>[4x]GSHMLFDFENDQVPSNIHFLNARASIETYTGINGEPSKGLKLAMQSKQHSYTGLAIVPEQPWDWSEFTSASLYFDIVSVGDHSTQFYLDVTDQNGAVFTRSIDIPVGKMQSYYAKLSGHDLEVPDSGDVNDLNLASGLRSNPPTWTS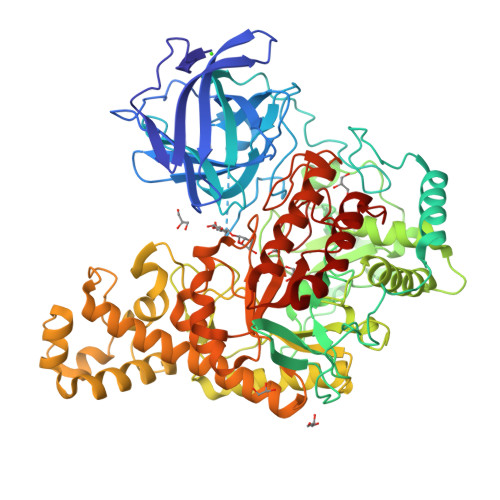DDRQFVWMWGVKNLDLSGIAKISLSVQSAMHDKTVIIDNIRIQPNPPQDENFLVGLVDEFGQNAKVDYKGKIHSLEELHAARDVELAELDGKPMPSRSKFGGWLAGPKLKATGYFRTEKINGKWMLVDPEGYPYFATGLDIIRLSNSSTMTGYDYDQATVAQRSADDVTPEDSKGLMAVSEKSFATRHLASPTRAAMFNWLPDYDHPLANHYNYRRSAHSGPLKRGEAYSFYSANLERKYGETYPGSYLDKWREVTVDRMLNWGFTSLGNWTDPAYYDNNRIPFFANGWVIGDFKTVSSGADFWGAMPDVFDPEFKVRAMETARVVSEEIKNSPWCVGVFIDNEKSFGRPDSDKAQYGIPIHTLGRPSEGVPTRQAFSKLLKAKYKTIAALNNAWGLKLSSWAEFDLGVDVKALPVTDTLRADYSMLLSAYADQYFKVVHGAVEHYMPNHLYLGARFPDWGMPMEVVKAAAKYADVVSYNSYKEGLPKQKWAFLAELDKPSIIGEFHIGAMDHGSYHPGLIHAASQADRGEMYKDYMQSVIDNPYFVGAHWFQYMDSPLTGRAYDGENYNVGFVDVTDTPYQEMVDAAKEVNAKIYTERLGSK{[(2,2-DIHYDROXY-ETHYL)-(2,3,4,5-TETRAHYDROXY-6-PHOSPHONOOXY-HEXYL)-AMINO]-METHYL}-PHOSPHONIC ACID | C9 H23 N O13 P2 | 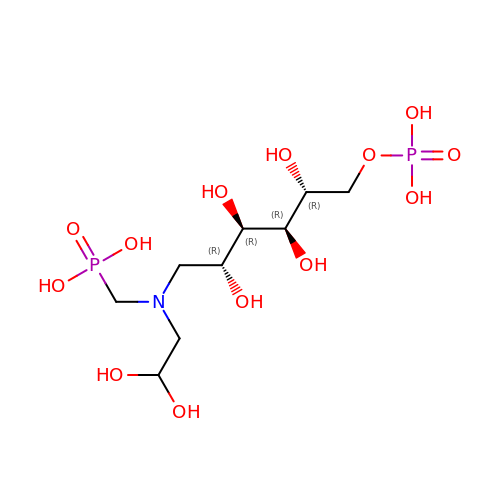ATILYNKCRYHYEP-SQEXRHODSA-N> SFMDRKEVVNIQT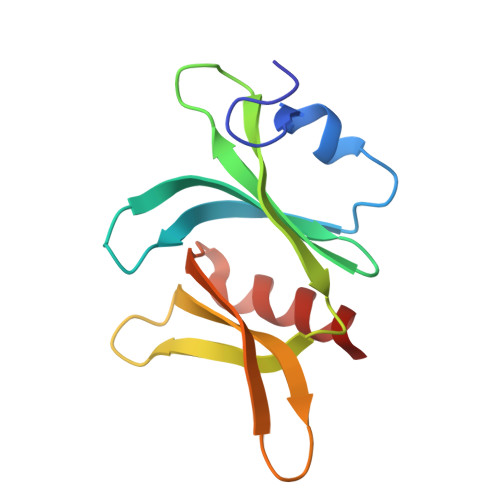WINKPDIKHHFPCKEVKESGHMFPSHLLVTATHMYCLREILSRKGLAYIQSRQALNSVVKITSKKKHPELITFKYGNSSASGIEILAIERYLIPNAGDATRAIKQQIMK>[6x]NSRTVLILCGDYMEDYEVMVPFQALQAFGITVHTVCPGKKAGDSCPTAVHDFCGHQTYFESRGHNFTLNATFDEVDLSKYDGLVIPGGRAPEYLALTASVVELVKEFSRSGKPIASICHGQLILAAA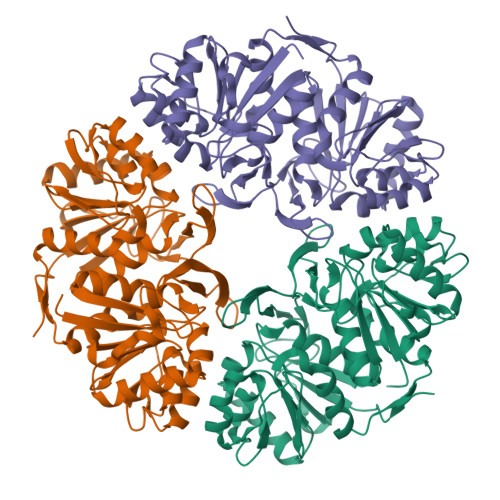DTVNGRKCTAYATVGPSLVAAGAKWVEPITPDVCVVDGSLITAATYEGHPEFIQLFVKALGGKITGANKRILFLCGDYMEDYEVKVPFQSLQALGCQVDAVCPEKKAGERCPTAIHDFEGDQTYSEKPGHTFALTTNFDDLVSSSYDALVIPGGRAPEYLALNEHVLNIVKEFMNSEKPVASICHGQQILAAAGVLKGRKCTAYPAVKLNVVLGGGTWLEPDPIDRCFTDGNLVTGAAWPGHPEFVSQLMALLGIQVSFH>SDEVRKNLMDMFRDRQAFSEHTWKMLLSVCRSWAAWCKLNNRKWFPAEPEDVRDYLLYLQARGLAVKTIQQHLGQLNMLHRRSGLPRPSDSNAVSLVMRRI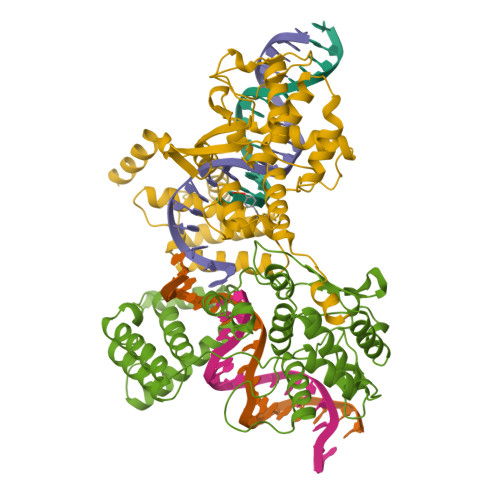RKENVDAGERAKQALAFERTDFDQVRSLMENSDRCQDIRNLAFLGIAYNTLLRIAEIARIRVKDISRTDGGRMLIHIGRTKTLVSTAGVEKALSLGVTKLVERWISVSGVADDPNNYLFCRVRKNGVAAPSATSQLSTRALEGIFEATHRLIYGAKDDSGQRYLAWSGHSARVGAARDMARAGVSIPEIMQAGGWTNVNIVMNYIRNLDSETGAMVRLLED[2x]> SMPPTVTVDRPFVVLIYDEKTRAVIFMGRVADPK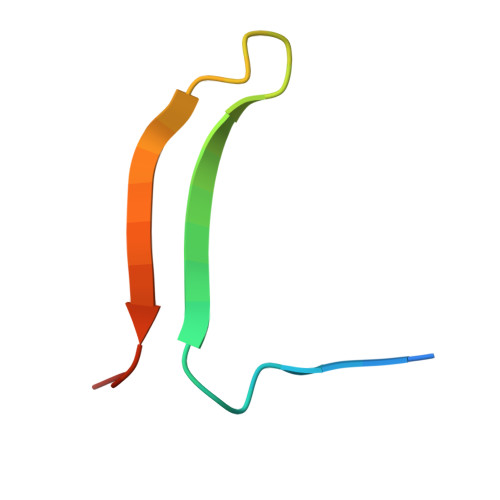Q>[6x]ADGNNIKAPIETAVKPPHRTEDNIRDEARRNRSNAVNPFSAKYVPFNAAPGSTESYSLDEIVYRSRSGGLLDVEHDMEALKRFDGAYWRDLFDSRVGKSTWPYGSGVWSKKEWVLPEIDDDDIVSAFEGNSNLFWAERFGKQFLGMNDL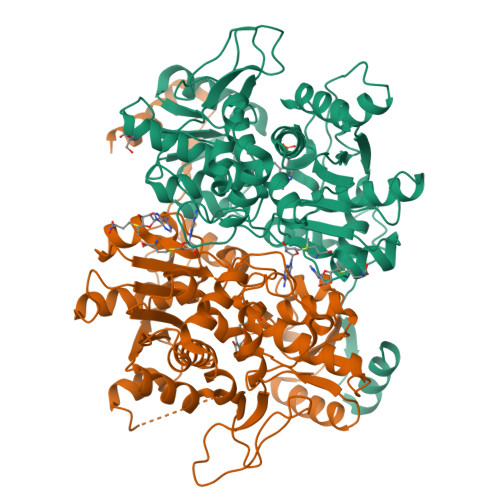WVKHCGISHTGSFKDLGMTVLVSQVNRLRKMKRPVVGVGCASTGDTSAALSAYCASAGIPSIVFLPANKISMAQLVQPIANGAFVLSIDTDFDGCMKLIREITAELPIYLANSLNSLRLEGQKTAAIEILQQFDWQVPDWVIVPGGNLGNIYAFYKGFKMCQELGLVDRIPRMVCAQAANANPLYLHYKSGWKDFKPMTASTTFASAIQIGDPVSIDRAVYALKKCNGIVEEATEEELMDAMAQADSTGMFICPHTGVALTALFKLRNQGVIAPTDRTVVVSTAHGLKFTQSKIDYHSNAIPDMACRFSNPPVDVKADFGAVMDVLKSYLGSNTLTS>[2x]RELTVGINGFGRIGRLVLRACME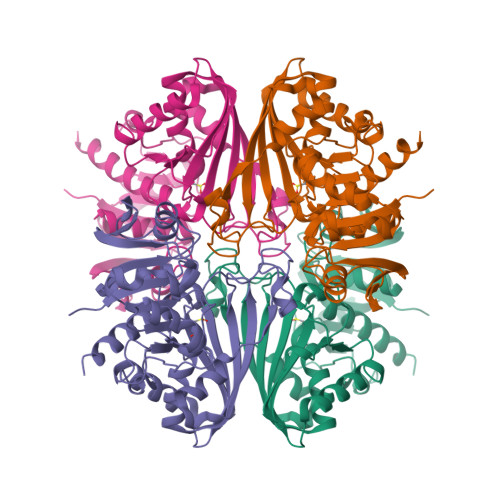KGVKVVAVNDPFIDPEYMVYMFKYDSTHGRYKGSVEFRNGQLVVDNHEISVYQCKEPKQIPWRAVGSPYVVESTGVYLSIQAASDHISAGAQRVVISAPSPDAPMFVMGVNENDYNPGSMNIVSNASCTTNCLAPLAKVIHERFGIVEGLMTTVHSYTATQKTVDGPSRKAWRDGRGAHQNIIPASTGAAKAVTKVIPELKGKLTGMAFRVPTPDVSVVDLTCRLAQPAPYSAIKEAVKAAAKGPMAGILAYTEDEVVSTDFLGDTHSSIFDAKAGIALNDNFVKLISWYDNEYGYSHRVVDLLRYMFSRDAE> MDECLPNSCLLGVHLVISTHSGPQIVYHYPPSNTAFLTNNPTKHQHLYGNHANLNKNTSTNKEEKLFNSGSTKTASQIALNESAKSYNTAITPSMTNTNTNNVTLPPTRSHANTVGSQSSIPAATNGVGYRKTDIEDTSRTFQYQETESETSSSGLSDSELSTDYLDISSDSFSISSSLSSSSLSSSPSSSSSSSPPQDGLSRTNSSFQSTDSMSPTSPQMIMENDSISVAESYLDSGTNNKSRAASKRSQNFFHKLSTKKSTDSKTHSPVRKLKSKPSQSTKKGNKLLKNTSNETDGNAFTGSCSISSKKSLSSTGEHNQELRNSSLNDTPGQSPHHYHHRYHHYHKNAATSQRNSHTQYDVEEEDMEVSAMLQDGKISMNEIFFEEENFQDINKILEFDNDFVAEFCSPEREMCNTRFEFTVDN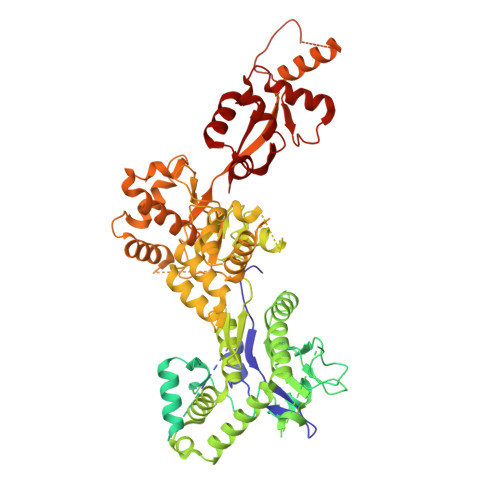FCFLGLPIHVDSQGRWRKSKHKNKTRSKRSSSTTTNISRKKSIASKISSLSENTLKKVNSGEADTVYDSNIGHEASTDTPNLRINTDVSGNEFEREKEDLGKNMNMFHVCFVMNPHLIEYNKRIDDMYQFVVTRLSLLLRYVQSKTSYISSECHIILKEKERVLKHSKTYQSIRGAGNKGKYLYQRILAKSSLARALTECVDKIQRNEIACLEINDDKVISLQIPIQNEFEKMPNFKLQPVLRGSYLTSILNMKFLEKSSLRIESQNRQNDQAQFSDTNNNIYRFGNNINSTGHCGAANVDDGDDNESNYYCDDNDDLLNYALLLLDEPNNIISSLETFSYQDDIGTIILKHLVRNIQPNIPLRSYRYLITDLLDNPSSLDDLTTETNSLESSILRSCALHLMYWRHARIVIPLSSKYTYIVSPLAPIQGYTIDDYKSTSQNDGNVKKMDDRENNKSGSDRVPLIYQNSMLFRSKFPSLPSLPIFLSLLSTDKPQAYSNIIPSREHKPVYLNALAWLIQYGYVTQLLTFINIRVDKHIKMAVDEDLEKEGFRKTNTARRPSMDYKKTDKKLDDEDGQSRDANASEACSGKNEGMQSNDNNKDVDEKDNENDSRVDDRDDNEIAIADEEEILHFEYDDPEMQHDYTIILEPERATAIEKRWLYRCIYGQPSDIQILFNKLLKYFNGKVPMELVIIKEEISRHDLKKLLNALDKYLIEIHHW> GSQMTRQARRLYVGNIPFGITEEAMMDFFNAQMRLGGLTQAPGNPVLAVQINQDKNFAFLEFRSVDETTQAMAFDGIIFQGQSLKIRRPHDYQPLPGMSENPSVYVPGVVSTVVPDSAHKLFIGGLPNYLNDDQVKELLTSFGPLKAFNLVKDSATGLSKGYAFCEYVDINVTDQAIAGLNGMQLGDKKLLVQRASVGAKN

A tightly controlled assembly among U2AF65, the pre-mRNA, and partner proteins sequentially identifies the 3′ splice site and promotes association of the spliceosome, which ultimately accomplishes the task of splicing. Initially U2AF65 recognizes the Py-tract splice site signal. Biochemical characterizations of U2AF65 demonstrated that tandem RNA recognition motifs (RRM1 and RRM2) recognize the Py tract. To investigate the structural basis for cognate U2AF65 recognition of a contiguous Py tract, we determined four crystal structures of U2AF651,2L bound to Py-tract oligonucleotides.

By sequential boot strapping, we optimized the oligonucleotide length, the position of a Br-dU, and the identity of the terminal nucleotide (rU, dU and rC) to achieve full views of U2AF651,2L bound to contiguous Py tracts at up to 1.5 Å resolution. The protein and oligonucleotide conformations are nearly identical among the four new U2AF651,2L structures. An extended conformation of the U2AF65 inter-RRM linker traverses across the α-helical surface of RRM1 and the central β-strands of RRM2 and is well defined in the electron density. The extensions at the N terminus of RRM1 and C terminus of RRM2 adopt well-ordered α-helices. Both RRM1/RRM2 extensions and the inter-RRM linker of U2AF651,2L directly recognize the bound oligonucleotide. Surprisingly, the RRM2 extension/inter-RRM linker contribute new central nucleotide-binding sites near the RRM1/RRM2 junction and the RRM1 extension recognizes the 3′-terminal nucleotide. The N- and C-terminal extensions of the U2AF65 RRM1 and RRM2 directly contact the bound Py tract. Rather than interacting with a new 5′-terminal nucleotide as we had hypothesized, the C-terminal α-helix of RRM2 instead folds across one surface of rU3 in the third binding site. There, a salt bridge between the K340 side chain and nucleotide phosphate, as well as G338-base stacking and a hydrogen bond between the backbone amide of G338 and the rU3-O4, secure the RRM2 extension.> ATLAFILYKYFPFG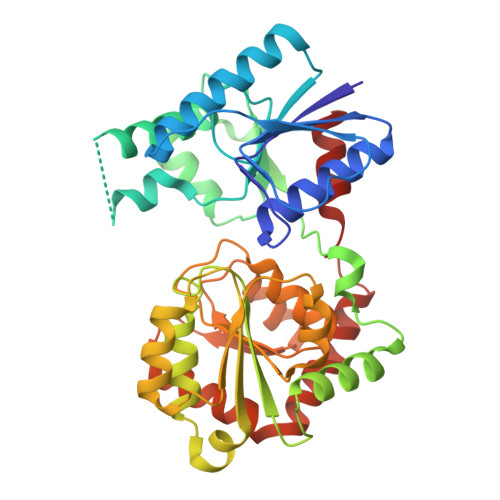GLQRDFMRIALECQRRGHDIRVYTLIWEGDVPDGFEVLVAPVRSIFNHRRNEKFTAWVRADLDRRPVQRVIGFNKMPGLDVYYAADACFEEKAQTLRNPLYRQWGRYRHFAGYERAVFDPASKTEILMISEVQQPLFVKHYGTQAERFHLLPPGISQDRRAPANAADVRAEFRREFGLEEDDLLLVQIGSGFKTKGLDRSLKALSALPKALRRRTRLIAIGQDDPKPFLLQIAALGLNDQVQILKGRSDIPRFLLGADLLIHPAYNENTGTVLLEALVSGLPVLVTDVCGYAHYIAEADAGRVLPSPFEQDSLNRLLAEMLEDAPARAAWSRNGLAYADHADLYSMPQRAADLILG>MSLINTKIKPFKNQAFKNGEFIEITEKDTEGRWSVFFFYPADFTFVCP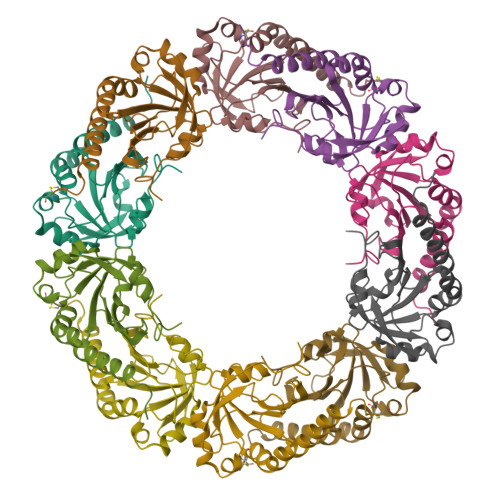TELGDVADHYEELQKLGVDVYAVSTDTHFTHKAWHSSSETIAKIKYAMIGDPTGALTRNFDNMREDEGLADRATFVVDPQGIIQAIEVTAEGIGRDASDLLRKIKAAQYVASHPGEVCPAKWKEGEATLAPSLD[5x]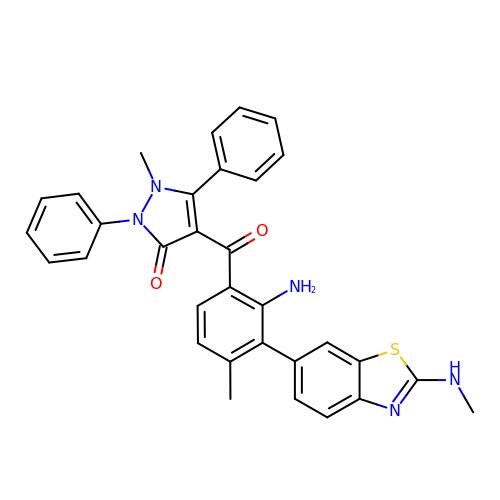4-{2-amino-4-methyl-3-[2-(methylamino)-1,3-benzothiazol-6-yl]benzoyl}-1-methyl-2,5-diphenyl-1,2-dihydro-3H-pyrazol-3-one | C32 H27 N5 O2 S | XUIZYNXJUPSUNY-UHFFFAOYSA-N> RGWVEICAADD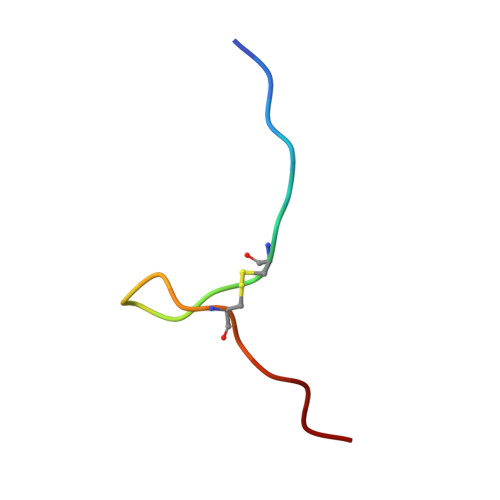YGRCLTEAQ>SRTDRLEVCREYQRGNCNRG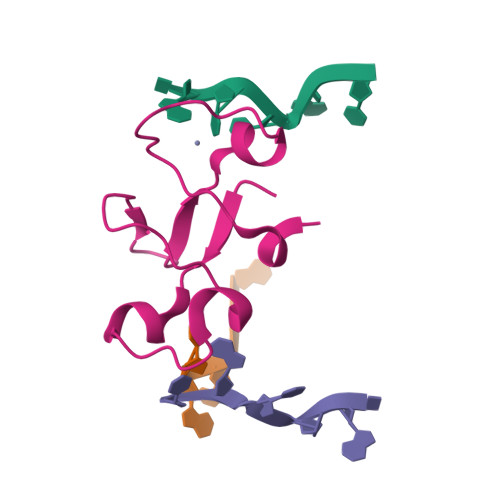ENDCRFAHPADSTMIDTNDNTVTVCMDYIKGRCSREKCKYFHPPAHLQAK[4x]N-[(4aS,6S,8aR)-2-amino-4a,5,6,7,8,8a-hexahydro-4H-3,1-benzothiazin-6-yl]-3-chlorobenzamide 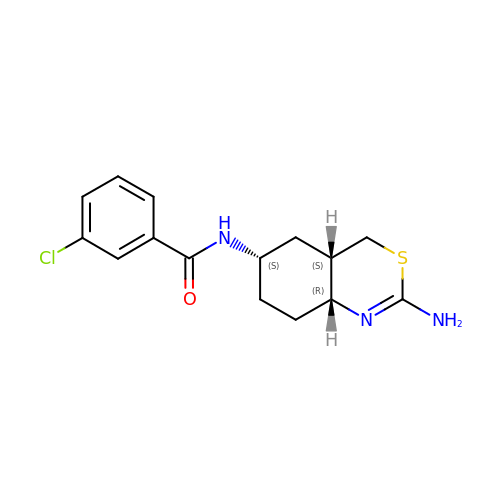| C15 H18 Cl N3 O S | TUSBLKXHGGIFCU-KGYLQXTDSA-N> MAPRGRRRPRPHRSEGARRSKNTLERTHSMKDKAGQKCKPIDVFDFPDNSDVSSIGRLGENEKDEETYETFDPPLHSTAIYADEEEFSKHCGLSLSSTPPGKEAKRSSDTSGNEASEIESVKISAKKPGRKLRPISDDSESIEESDTRRKVKSAEKISTQRHEVIRTTASSELSEKPAESVTSKKTGPLSAQPSVEKENLAIESQSKTQKKGKISHDKRKKSRSKAIGSDTSDIVHIWCPEGMKTSDIKELNIVLPEFEKTHLEHQQRIESKVCKAAIATFYVNVKEQFIKMLKESQMLTNLKRKNAKMISDIEKKRQRMIEVQDELLRLEPQLKQLQTKYDELKERKSSLRNAAYFLSNLKQLYQDYSDVQAQEPNVKETYDSSSLPALLF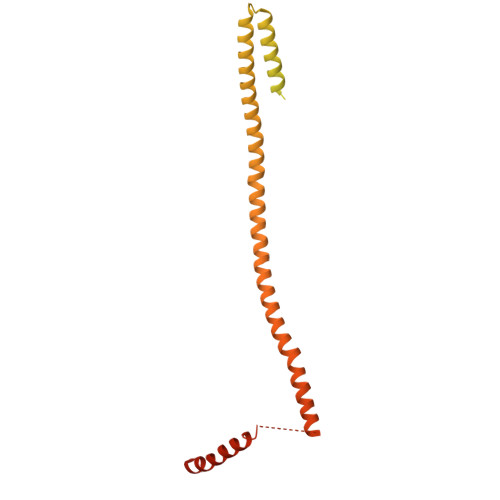KARTLLGAESHLRNINHQLEKLLDQG> AU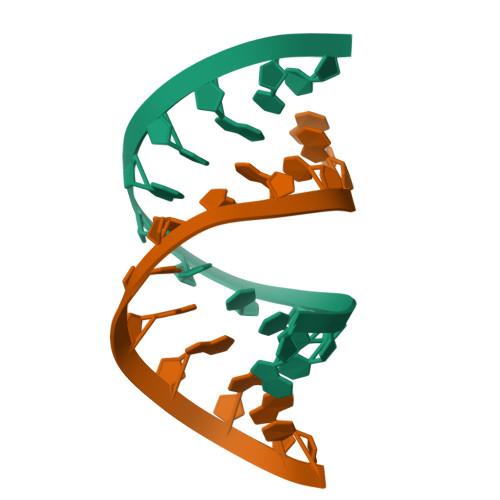CCCCCGUGCC;> GGUGCGGGGGAU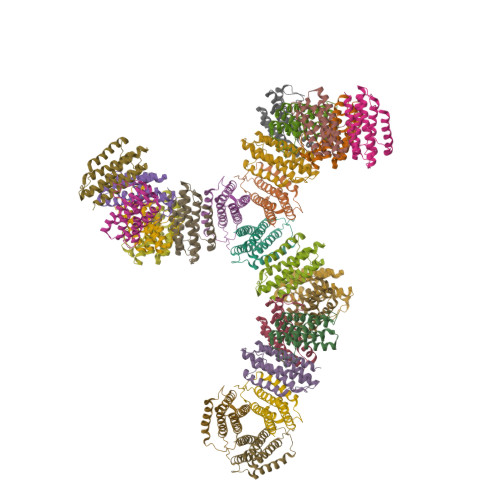> MFTRRGDQGETDLANRARVGKDSPVVEVQGTIDELNSFIGYALVLSRWDDIRNDLFRIQNDLFVLGEDVSTGGKGRTVTLEMILYLVERVTEMKAEIGKIELFVVPGGSVESASLHMARAVSRRLERRIKAASRLTEINDNVLLYAAMLSSILFMHALISNKRLNIPEKIWSIHRVSLEHHHHHH> L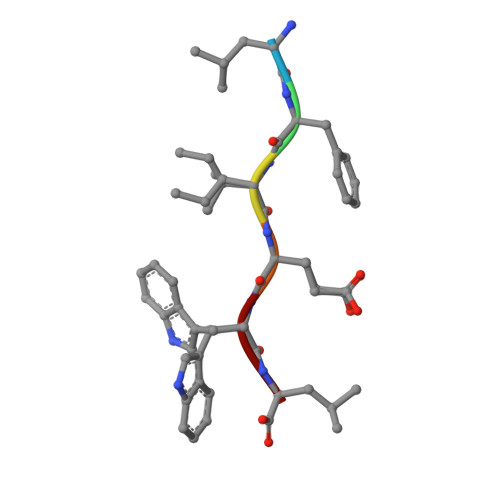FIEWL>[4x]UAGCUCC;>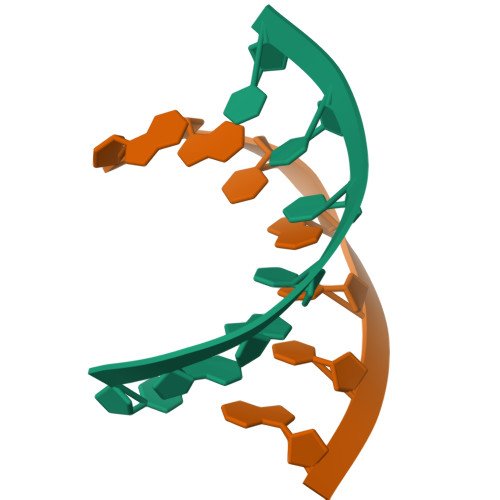GGUGCUA[4x]> MALEEIRPKEVYLDRKLLTLEDKELGSGNFGTVKKGYYQMKKVVKTVAVKILKNEANDPALKDEL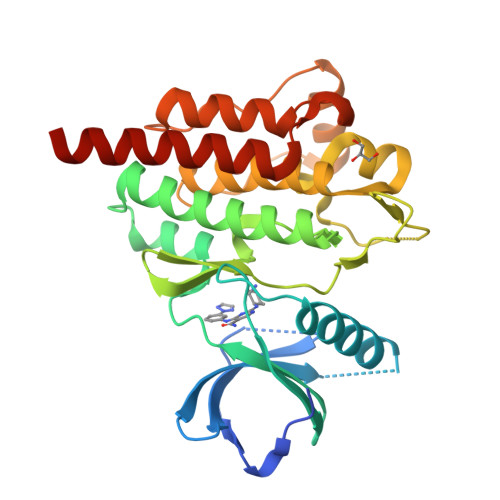LAEANVMQQLDNPYIVRMIGICEAESWMLVMEMAELGPLNKYLQQNRHVTDKNIIELVHQVSMGMKYLEESNFVHRDLAARNVLLVTQHYAKISDFGLSKALRADENYYKAQTHGKWPVKWYAPECINYYKFSSKSDVWSFGVLMWEAFSYGQKPYRGMKGSEVTAMLEKGERMGCPAGCPREMYDLMNLCWTYDVENRPGFAAVELRLRNYYYDVVNHHHHHHH> DAASVYTLPAGADFLMCYSVAEGYYS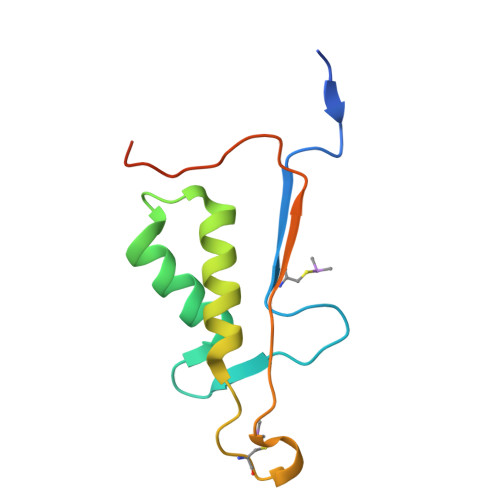HRETVNGSWYIQDLCEMLGKYGSSLEFTELLTLVNRKVSQRRVDFCKDPSAIGKKQVPCFASMLTKKLHFFPKSNRHHHHHH> GSMGNLAEKMYKAGNAMYRKGQYTIAIIAYTLALLKDPNNAEAWYNLGNAAYKKGEYDEAIEAYQKALELDPNNAEAWYNLGNAYYKQGDYDEAIEYYKKALRLDPRNVDA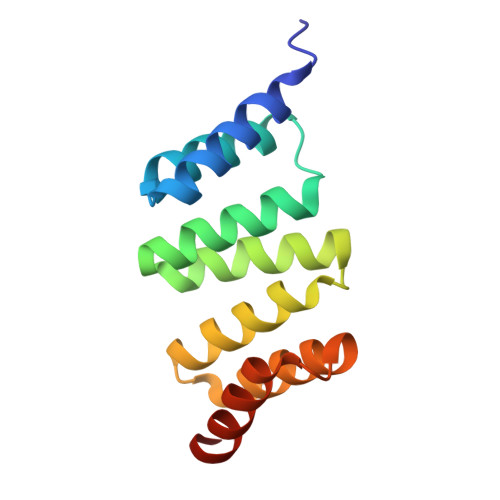IENLIEAEEKQGAS>KGLENPLPERPREKEEPVVRETGEVVDCHLSDMLQQLHSVNASKPSERGLVRQEEAEDPACIPIFWVSKWVDYSDKYGLGYQLCDNSVGVLFNDS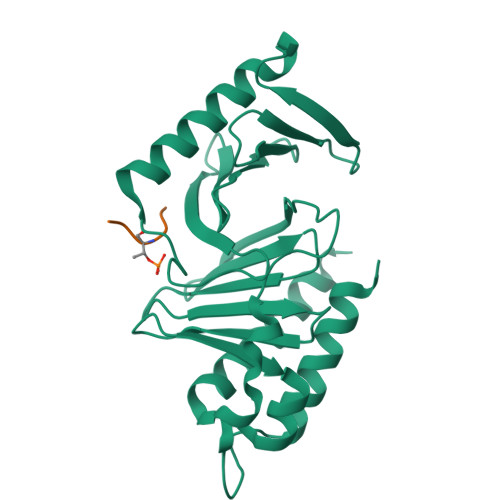TRLILYNDGDSLQYIERDGTESYLTVSSHPNSLMKKITLLKYFRNYMSEHLLKAGANITPREGDELARLPYLRTWFRTRSAIILHLSNGSVQINFFQDHTKLILCPLMAAVTYIDEKRDFRTYRLSLLEEYGCCKELASRLRYARTMVDKLLSSRSASNRLKAS[3x];>[3x]MQSTPL> MCGDQSDHVLQHWTVDISIDEHEGLTRAKARLRWREKELVGVGLARLNPADRNVPEIGDELSVARALSDLGKRMLKVSTHDIEAVTHQPAR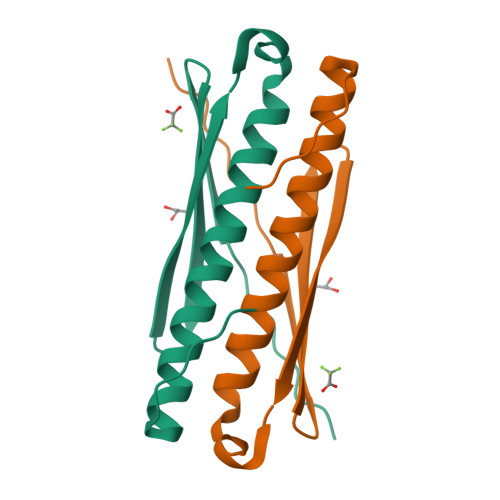LLY ADP-ribosylation is a reversible post-translational modification involved in various cellular activities. Removal of ADP-ribosylation requires (ADP-ribosyl)hydrolases, with macrodomain enzymes being a major family in this category. Further analyses reveal DUF4804 as a class of MavL-like macrodomain enzymes whose representative members show unique selectivity for mono-ADP-ribosylated arginine residue in synthetic substrates. Crystal structures of several proteins in this class provide insights into arginine specificity and a shared mode of ADP-ribose interaction distinct from previously characterized macrodomains.

Two of the representative proteins in this group, CG2909, and CG3568, are from Drosophila melanogaster, indicating potential evolutionary connections between the prokaryotic effector and the eukaryotic proteins. Encouraged by the clearly detectable ADPR-Ub hydrolytic activity of the two metazoan proteins, we solved their crystal structures in the ADPR-bound forms (ADPR-bound CG290912-498 at 2.28 Å and the ADPR-bound CG356825-508 at 2.00 Å). The ADPR interactions in both CG2909 and CG3568 are similar to those observed in MavL, with di-phosphate-binding loops and catalytic loops matching the sequence motifs identified from our search. In addition, water molecules equivalent to w4 in MavL can be found in both structures with distances of 3.4 Å (in CG2909) and 3.3 Å (in CG3568), suggesting that this macrodomain class likely employs a similar catalytic mechanism. Adenosines in MavL, CG2909, and CG3568 are sandwiched between two residues and stabilized by π-π (in MavL) or π-π and π-cation (in CG2909 and CG3568) interactions. In MavL, the adenosine was stabilized by π-π stacking interaction provided by two aromatic residues (H142 and Y265), whereas in the two Drosophila proteins, a π-cation interaction involving an arginine (R198 in CG2909 and R209 in CG3568) replaces the imidazolium stacking. In Arg-specific macrodomains, the core β-strand connectivity appears to be the same, yet some distinct differences are observed: In both CG2909 and CG3568, expansion of the variable regions from β7 to β9 (compared to β4–β5 in MavL) and the additional β12–β13 were observed. Interestingly, CG2909, CG3568, and Larg1 all harbor a hydrophobic residue (F137 in CG2909, F148 in CG3568, and V77 in Larg1) equivalent to F105 in MavL in their insertions. Note that MavL, CG3568, and Larg1 harbor a glutamate residue (E107 in MavL, E237 in CG3568, and E160 in Larg1) at the same position that does not interact directly with the distal ribose. On the other hand, our study also tapped into the protein-level specificity: MavL interacts with Ub and effectively removes ADPR from ADPR-Ub, whereas Larg1, CG2909, and CG3568 exhibited rather weak activity hydrolyzing ADPR-Ub.

>[4x]GPLGSWPGKRTNLPENAFTQRMLQECGQMAKPDASVDLDNFKAISEQSPAEFGIDSCRVKAQPEDRSDRIREQIASAYPVIHERTLLLFISFLEHKLTFGSEQEKAIYKDMTVVDLVQRLLAKRCVWFFGANDYYRTMQGNIGNEGFEAVGTPAEKEPLTLTSVLSYDEIKLSALLYVSCHSEFINNGSRVNGGEVLQNKDTIEREGVVIGLIGARFERPDVMEYQDIMITKTQNTEANGYGFDLEQISSETVTPASDLRRIWREFYEEPRDFIYADTPYDTTRFEEVSQGIFDHQVMRKRYAISFDTLLLEAQDRAFKAGKPAYIHVVGIGLGVWKAARQQERTFLESFEGRLRALGERLSHIGVVHFSWFHLACVGSLHDGAIIPVDKHPQGGIRIRNSVRNPGDKLTEDMLPVVTYAWDGNALPGNEFWANMLISTGDPAAACSTLISELQNPHINVHYMNGANLHIASVEHGLLHVGDYARRLIV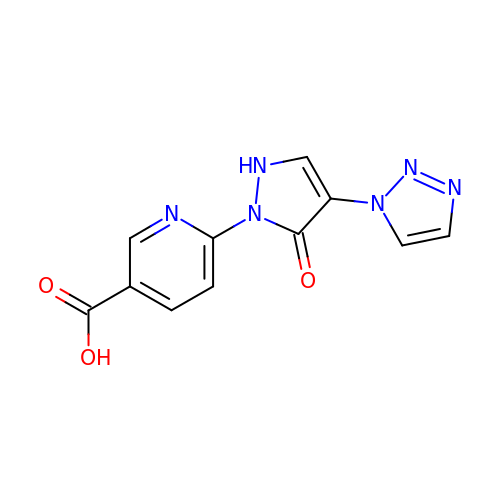6-(5-oxo-4-(1H-1,2,3-triazol-1-yl)-2,5-dihydro-1H-pyrazol-1-yl)nicotinic acid | C11 H8 N6 O3 | MRJSXXCYZJCFSP-UHFFFAOYSA-N>[4x]MAQPIVFYDIPSNERIKHSPWSPNTWKIRYALNYKGLKYKTEWVEYPDIAGVVQKLGGKPTEKTPDGRDHYTLPVIYDPNTKKVVEDSAAIAKYLDETYPDTPKLFPAGTDAFQAAFLDFAWPVLGFPVFMLVILDTANSLLPRSHDYFRSTREQKFGKKLEELATEEEWAKVEAGLAKLKGYLDANGK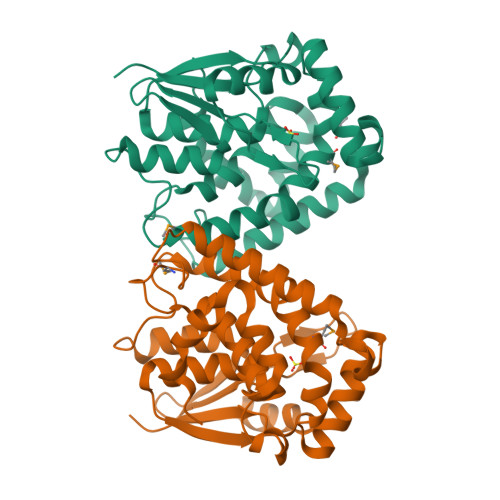GNDLLLMGAQGGITYSDIQIASFFVWAKIIWGEGSEKWKRLISLHDGKWAQFYAQFTKFEQVDV>GSDILRYLDFSNSSGQIISTVYPFYVQMNYFAEIKYYITYHYEAKKNYDEAYNQSVNPLMSSIQNQINSCVPKKAALEKTIFVLEYPENHNINLSNYEAKHNEYKQQLDAYKNCVQANMESYTDRMSKFNEKIYSILNSVKCTDACETDTYEIMLEIYVERVKEVNHNNYVNYLSTLKASLQLGVTLMLKVKQEIDNNVTISAINFLQEEMLDIITIGEAHTGKIIHGKENVLKLQNNNIPPQVPLSTLKKLYFDSANFYATYKFSLKRADTTTAALK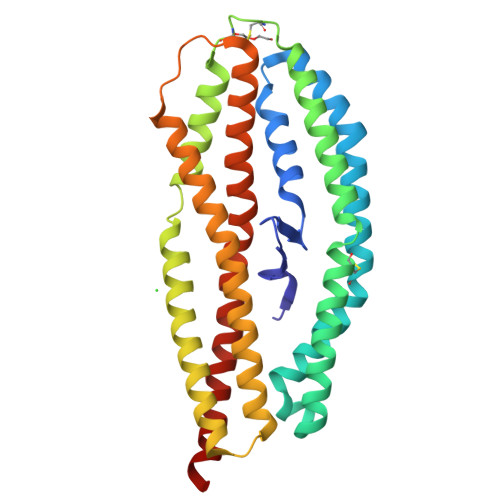EKGKLLANLYNKLITYVSEK[2x]> MAYPESLKAHLQGGVTTLARAWALARADGRVLGFTDHDVVLRFDGISFEPGSGMTAKAVLQGTGLSVDNTESYGALSSEAITEADLLAGRYDGAAVTVWLVNWADPAMRAVIFRGHLGEVSRGAGAFTAELRGLTA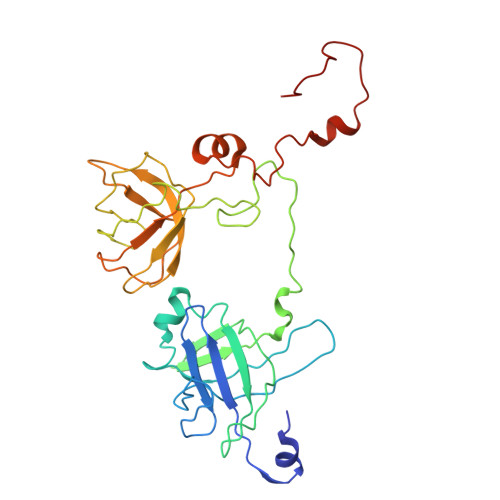ALGQEQGRIYHPRCAAVLGDGRCRFDLTKDGYALEAALGGVDEAVVLRLAEGAGFEDRWFEKGRLVVLDGAAAGLIGVVKNDRLQADGSRLIELWQRLGANPVAGDRVRIEPGCDKRAGTCRLKFDNFLNFRGFPHIPGEDWMVSYPVQSGTNDGGSLFR> SMFLPPPECPVFEPSWEEFADPFAFIHKIRPIAEQTGICKVRPPPDWQPPFACDVDKLHFTPRIQRLNELEAQTRLKLGGGGARDYTLRTFGEMADAFKSDYFNMPVHMVPTELVEKEFWRLVSTIEEDVTVEYGADIASKEFGSGFPVRDGKIKLSPEEEEYLDSGWNLNNMPVMEQSVLAHITADICGMKLPWLYVGMCFSSFCWHIEDHWSYSINYLHWGEPKTWYGVPGYAAEQLENVMKKLAPELFVSQPDLLHQLVTIMNPNTLMTHEVPVYRTNQCAGEFVITFPRAYHSGFNQGFNFAEAVNFCTVDWLPLGRQCVEHYRLLHR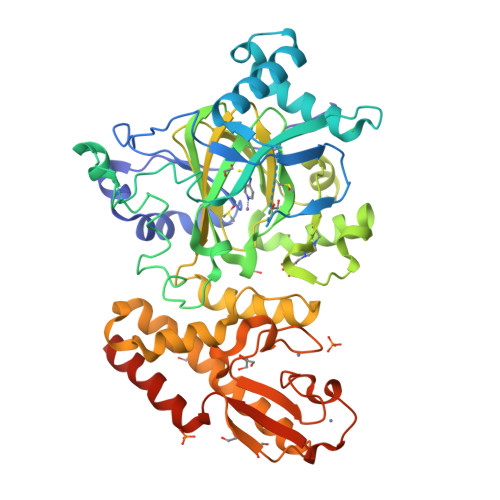YCVFSHDEMICKMASKADVLDVVVASTVQKDMAIMIEDEKALRETVRKLGVIDSERMDFELLPDDERQCVKCKTTCFMSAISCSCKPGLLVCLHHVKELCSCPPYKYKLRYRYTLDDLYPMMNALKLRAESYNEWALNVNEALEAKI> MRLSYEALEWRTPIENSTEPVSLPPPPPFFGQERAREALELAIRGGFHAYLVGPPSLGKHEALLAYLSTQSVETPPDLLYVPLSERKVAVLTLPSGQEIHLAEAVEGLLLEVNRLDELFRQGSFLREKTQLEARFKEAREQQLEALRREAQEAGFALSTNGERLELTGPGPVPAELSARLEEVTLGSLAASAELEVALRRLRRDWALHYLNNRFEPLFQRFPQARAYLEALRARLARYAETGEPLDPAQWRPNLLTSSSSGTPPPIVYEPYATAPRLFGRLDYLVDRGVWSTNVSLIRPGAVHRAQGGYLILDALSLKREGTWEAFKRALRNGQVEPVTEPQAPAGLEVEPFPIQMQVILVGTPEAFEGLEEDPAFSELFRIRAEFSPTLPASPENCTALGGWLLAQGFQLTQGGLTRLYDEARRMAEQRDRMDARLVEIRALAEEAAVLGGGLLTAESVEQAIAAREHRSFLSEEEFLRAVQEGVIRLRTTGRAVGEVNSLVVVEAAPYWGRPARLTARAAPGRDHLISIDREAGLGGQIFHKAVLTLAGYLRSRYIEHGSLPVTISLAFEQNYVSIEGDAAGLAELVAALSAIGNLPLRQDLAVTGAVDQTGKVLAVGAINAKVEGFFRVCKALGLSGTQGVILPEANLANLTLRAEVLEA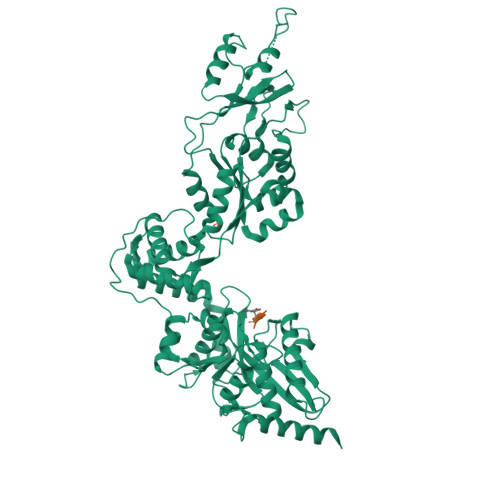VRAGQFHIYAVETAEQALEILAGARMEGFRGLQEKIRAGLEAFARLEEGHDKEDREKLAAALEHHHHHH;> AVYA> QECSLQSCTQHQPYVVDDPCPIHFYSKWYIRVGARKSAPLIELCVDEAGSKSPIQYIDIGNYTVSCSPFTINCQEPKLGSLVVRCSFYEDFLEYHDVRVVLDFI

ORF8 is a viral immunoglobulin-like (Ig-like) domain protein encoded by the severe acute respiratory syndrome coronavirus 2 (SARS-CoV-2) RNA genome. It tends to evolve rapidly and interfere with immune responses. The full-length SARS-CoV-2 ORF8 is composed of a signal peptide (residues 1-15) and an Ig-like domain (residues 16-121). Herein, we determined the crystal structures of SARS-CoV-2 ORF8 (S84) (one of the epidemic isoforms) and the bat coronavirus RaTG13 ORF8 variant at 1.62 Å and 1.76 Å resolution, respectively.

The Ig-like domain of SARS-CoV-2 ORF8 (S84) forms a “β-sandwich” that comprises two β-sheets and an additional β-hairpin. The smaller sheet is composed of three antiparallel strands (βB, βD, and βE), while the larger sheet is formed by five twisted strands (βA, βC, βC’, βF, βG) with loops. The protruding β-hairpin exists between strands βC’ and βD, consisting of strands βI1 and βI2. Of note, intramolecular disulfide bonds, including Cys25-Cys90, Cys37-Cys102, and Cys61-Cys83, contributed to stabilizing the β-sheet structure into an irregular β-sandwich fold. The electron density of residue Cys20 suggests that a potential intermolecular disulfide bond exists between two adjacent symmetric units. In detail, the SARS-CoV-2 ORF8 (S84) dimer is linked by an intermolecular disulfide bond formed between the two Cys20 residues of molecule A and A’. The residues from 62 to 77 in SARS-CoV-2 ORF8 (S84) assemble more tightly than their equivalent in RaTG13 ORF8, featuring a maximum 21.4 Å shift. In ORF8(S84), however, the closest distance between the two 71 - 75 loops is 2.7 Å, which occurs at the side chain of the two Asp75 and may not help SARS-CoV-2 ORF8 (S84) to form a dimer with this interface. By contrast, C20A and C20K mutants could not form a stable dimer in the absence of the reducing reagent. Thus, these data suggest that the SARS-CoV-2 ORF8(S84) form an inter-chain disulfide bond at Cys20. The mild disease outcome related S84 variant of the ORF8 protein demonstrates weaker binding ability with CD14+ monocytes, indicating that the ORF8 variants may adjust different degrees of inflammation by modulating monocyte recognition of viral antigens.(2S)-2-[(2-{3-[(2,4-diamino-6-ethylpyrimidin-5-yl)oxy]propoxy}phenyl)methyl]-3-fluoropropanoic acid | C19 H25 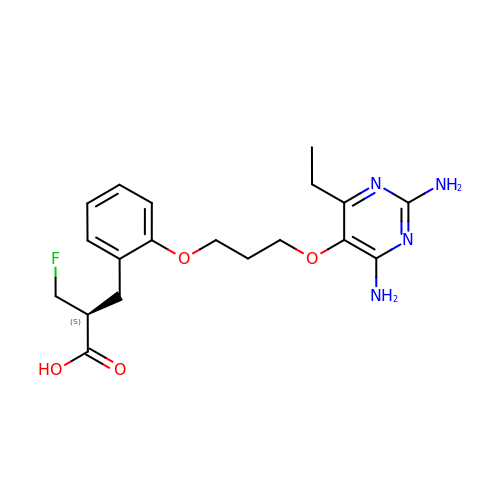F N4 O4 | CDIUQIVTNPRVDS-CYBMUJFWSA-N>STAGKVIKCKAAVLWEEKKPFSIEEVEVAPPKAHEVRIKMVATGICRSDDHVVSGTLVTPLPVIAGHEAAGIVESIGEGVTTVRPGDKVIPLFTPQCGKCRVCKHPEGNFCLKNDLSMPRGTMQDGTSRFTCRGKPIHHFLGTSTFSQYTVVDEISVAKIDAASPLEKVCLIGCGFSTGYGSAVKVAKVTQGSTCAVFGLGGAGLSVIMGCKAAGAARIIGVDINKDKFAKAKEVGATECVNPQDYKKPIQEVLT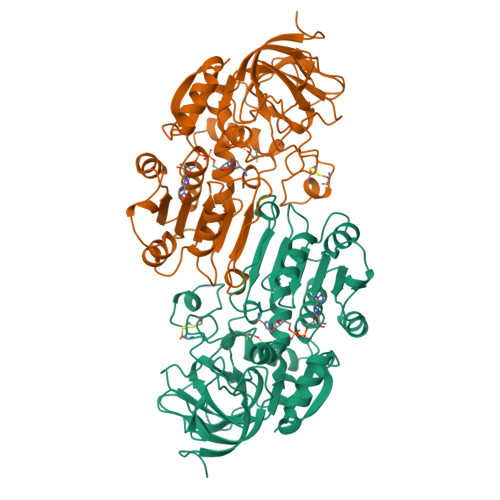EMSNGGVDFSFEVIGRLDTMVTALSCCQEAYGVSVIVGVPPDSQNLSMNPMLLLSGRTWKGAIFGGFKSKDSVPKLVADFMAKKFALDPLITHVLPFEKINEGFDLLRSGESIRTILTF[4x]> SQVTKTPRSNYTGPIVVDPLTRIEGHLRIEVEVEGGVIKEARSCATLFRGIETILKGRDPRDAQHFTQRTCGVCTYTHALASTRCLEDAINKPIPANATYIRNLVLGNQFMHDHLVHFYHLHALDFVDVTSALLADPAKAAKLANSISPRKATTEEFAAVQAKLKTFVASGQLGPFTNAYFLGGHEGYYMDPEANLVCTAHYLQALRAQVEVAKGMAVFGAKNPHTQFTVAGGVTCYEALTPERIKQFRELYVKARAFIEEVYIPDLLLVASYYKDWGKIGGTNNFMAFGEFPAPGGERDLNSRWYKPGVIYDRKVGSVQPFDPSKIEEHVRHSWYEGKARAPFEGETNPHFTFMGDTDKYSWNKAPRYDGHAVETGPLAQMLVAYGHNHKTIKPTIDAVLGKLNLGPEALFSTLGRTAARGIQTLVIAQQMENWLNEYENNIVKDKQIVEDYAV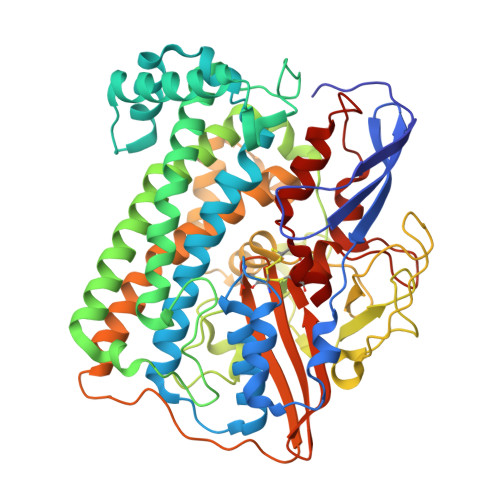PTSARGVGFADVSRGGLSHWMTIEDGKIDNFQLVVPTTWNLGPRDDKGVPSAAEAALVGTPVADPKRPVEILRTIHSFDPCIACSTH> MTIDQKNTNIDPRFPHHHPRPQSFWEARAKALESLLIEKGHLSSDAIERVIKHYEHELGPMNGAKVVAKAWTDPAFKQRLLEDSETVLRELGYYGLQGEHIRVVENTDTVHNVVVCTLCSCYPWPLLGLPPSWYKEPAYRARVVKEPRQVLKEFGLDLPDSVEIRVWDRSSEIRFMVLPQRPEGTEGMTEEELAKLVTRDSMIGVAKIEPPKVTVG;> MNGIHDVGGMDGFGKVMYVKEEEDIYFTHDWERLAFGLVAGCKAQGLGMKAFDEFRIGIELMRPVDYLTSSYYGHWIATVAYNLVDTGVLDEKELDERTEVFLKKPDTKIPRREDPALVKLVEKALYDGLSPLREISASPRFKVGERIKAKNIHPTGHTRFPRYARDKYGVIDEVYGAHVFPDDAAHRKGENPQYLYRVRFEAEEL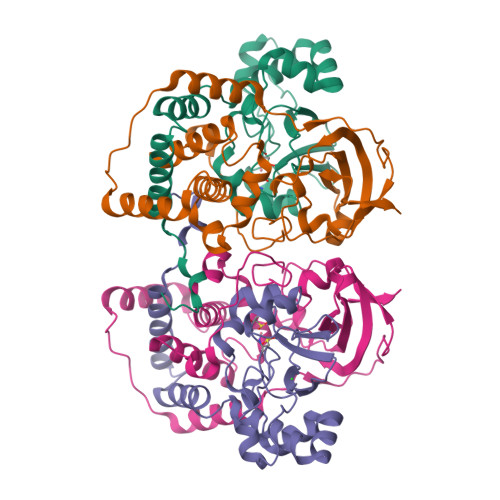WGYKQKDSVYIDLWESYMEPVSH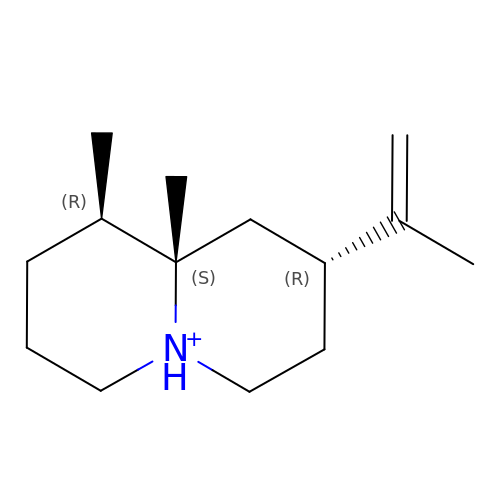(1R,5R,8R,9aS)-1,9a-dimethyl-8-(prop-1-en-2-yl)octahydro-2H-quinolizinium | C14 H26 N | XJMHVRNRJICXTC-MCIONIFRSA-O> GLPTMNTPGSNQFLTSDDFQSPCALPNFDVTPPIHIPGEVKNMMELAEIDTLIPMNAVDGKVNTMEMYQIPLNDNLSKAPIFCLSLSPASDKRLSHTMLGEILNYYTHWTGSIRFT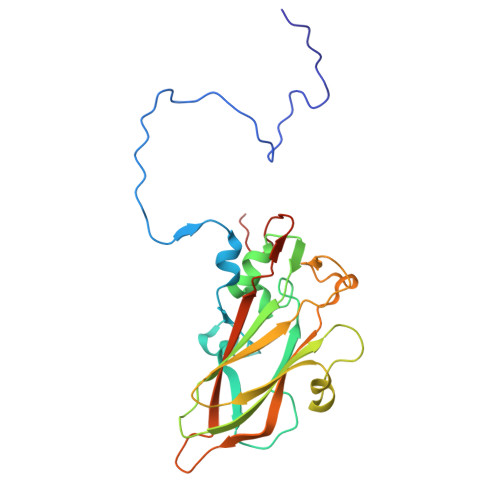FLFCGSMMATGKLLLSYSPPGAKPPTNRKDAMLGTHIIWDLGLQSSCSMVAPWISNTVYRRCARDDFTEGGFITCFYQTRIVVPASTPTSMFMLGFVSACPDFSVRLLRDTPHISQSKLIGRTQ Helicase E5 is a multi-domain protein; its primer synthesis and DNA unwinding activity are required for genome uncoating and DNA replication of MPXV. MPXV E5 is encoded by the E5R gene, the mature protein is 785 amino acids (aa) in length. MPXV E5 can be divided into 6 domains: the AEP domain, the ZnD domain (Zinc-binding domain), the D5N domain (a domain associated with D5-type helicases), the Linker, the SF3 Helicase domain, and the C-Tail. MPXV E5 belongs to the SF3 helicase superfamily, which normally forms hexamer and unwinds DNA with 3′- to 5′ polarity.

No crystal grew for AEP-ZnD, but one high-resolution AEP structure was determined (1.65 Å). Supported by the low RMSD value (0.6 Å), the overall foldings of the AEP domains are very similar in the crystal and cryo-EM structures. No DNA template or RNA product was observed, but clear electron densities confirmed that two Mg2+ ions (common factor of DNA and RNA polymerase) and one pyrophosphate group (PPi) were captured in the AEP structure. Since no PPi was included in the crystallization sample, the observed PPi should be produced by the AEP-catalyzed de novo synthesis reaction. In addition to the side chains of Asp70, Asp72 and Asp170, the A-site Mg2+ ion also coordinates with three water molecules. The B-site Mg2+ ion coordinates with the side chains of Asp70 and Asp72, two water molecules, and two oxygen atoms of PPi. Besides coordination with Mg2+ ion, the conformation of PPi was further stabilized by H-bond interactions with the side chains of Lys130, Ser132, His134, Arg181, Lys187, and His197. PPi in the MPXV E5 structure well mimics the β- and γ-phosphate groups of the incoming site (E-site) dATP in the MsCAPP structure. The similar structural arrangements suggested that the AEP domain of MPXV E5 follows the conserved two-cation-assisted, in-line attacking mechanism in catalysis, in which A-site cation activates the initiating site (I-site) NTP (or dNTP) by removing the proton from the 3′-OH group and B-site cation facilitates the reaction by increasing the electrophilicity of the phosphorus center. The de novo primer synthesis activity can be implicated by the PPi molecule observed in the crystal structure of the AEP domain of MPXV E5.

> MDAAIRGNDVIFVLKTIGVPSACRQNEDPRFVEAFKCDELERYIDNNPECTLFESLRDEEAYSIVRIFMDVDLDACLDEIDYLTAIQDFIIEVSNCVARFAFTECGAIHENVIKSMRSNFSLTKSTNRDKTSFHIIFLDTYTTMDTLIAMKRTLLELSRSSENPLTRSIDTAVYRRKTTLRVVGTRKNPNCDTIHVMQPPHDNIEDYLFTYVDMNNNSYYFSLQ> GSVCPQGKYIHPQDNSICCTKCHKGTYLYNDCPGPGQDTDCRE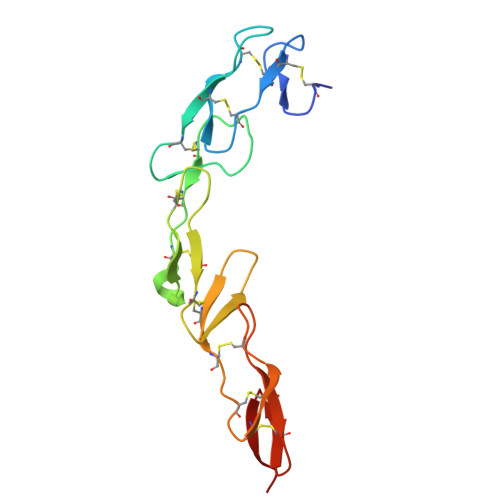CESGSFTASENHLRHCLSCSKCRKEMGQVEISSCTVDRDTVCGCRKNQYRHYWSENLFQCFNCSLCLNGTVHLSCQEKQNTVCTCHAGFFLRENECVSSSN> GAMATGDERFYAEHLMPTLQGLLDPESAHRLAVRFTSLGLLPRARFQDSDMLEVRVLGHKFRNPVGIAAGFDKHGEAVDG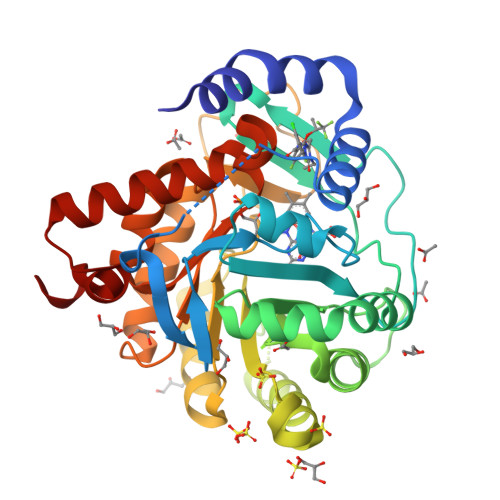LYKMGFGFVEIGSVTPKPQEGNPRPRVFRLPEDQAVINRYGFNSHGLSVVEHRLRARQQKQAKLTEDGLPLGVNLGKNKTSVDAAEDYAEGVRVLGPLADYLVVNVSSPNTAGLRSLQGKAELRRLLTKVLQERDGLRRVHRPAVLVKIAPDLTSQDKEDIASVVKELGIDGLIVTNTTVSRPAGLQGALRSETGGLSGKPLRDLSTQTIREMYALTQGRVPIIGVGGVSSGQDALEKIRAGASLVQLYTALTFWGPPVVGKVKRELEALLKEQGFGGVTDAIGADHRR5-[3-(2-methoxy-5-oxidanyl-phenyl)-1H-pyrrolo[2,3-b]pyridin-5-yl]-N,N-dimethyl-pyridine-3-carboxamide | C22 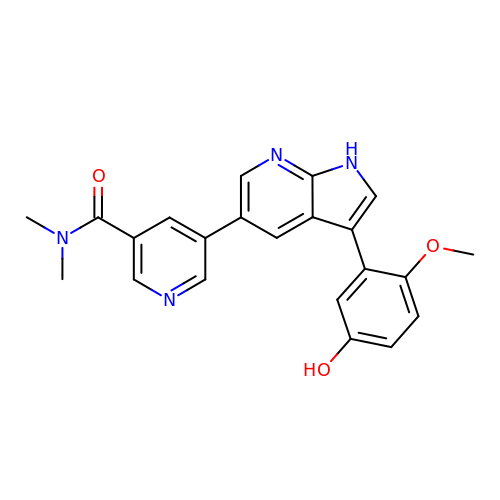H20 N4 O3 | LEFHTGQOJNMOKU-UHFFFAOYSA-N> XDDY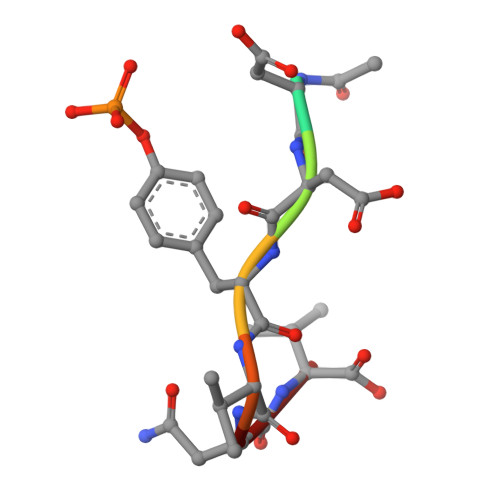VNV> GSHMTPAFNKPKVELHVHLSGAIKPETILYFGKKRGIALPADTVEELRNIIGMDKPLSQPGTLAKWDYYMPVIAGCREAIKRIAYEFVEMKAKEGVVYVEVRYSPHLLANSKVDPMPWNQTEGDVTPDDVVDLVNQGLHEGEQAFGIKVRSILCCMRHQPSWSLEVLELCKKYNQKTVVAMDLIGDETIEGSSLFPGHVEAYEGAVKNGIHRTVHAGEFGSPEVVREAVDILKTERVGHGYHTIEDEALYNRLLKENMHFEVCPWSSYLTGAWDPKTTHAVVRFKNDKANYSL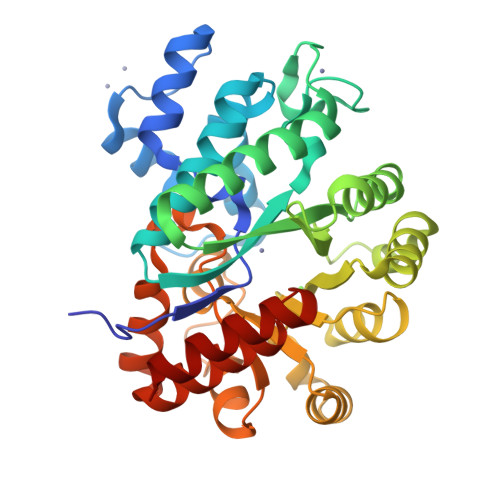NTDAPLEFKSTLDTDYQMTKKDMGFTEEEFKRLNINAAKSSFLPEEEKKELLERLYREYQ>AANPYERGPAPTNASIEA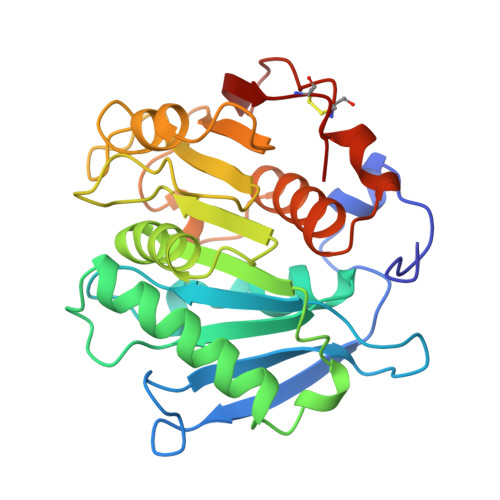SRGPYATSQTSVSSLVASGFGGGTIYYPTSTADGTFGAVVISPGFTAYQSSIAWLGPRLASQGFVVFTIDTNTTLDQPDSRGRQLLSALDYLTQRSSVRTRVDATRLGVMGHSMGGGGSLEAAKSRTSLKAAIPLTGWNTDKTWPELRTPTLVVGADGDTVAPVATHSKPFYESLPGSLDKAYLELRGASHFTPNTSDTTIAKYSISWLKRFIDSDTRYEQFLCPIPRPSLTIAEYRGTCPHTS[2x]>[2x]FACKTANGTAIPIGGGSANVYVNLAPAVNVGQNLVVDLSTQIFCHNDYPETITDYVTLQRGSAYGGVLSSFSGTVKYNGSSYPFPTTSETPRVVYNSRTDKPWPVALYLTPVSSAGGVAIKAGSLIAVLIL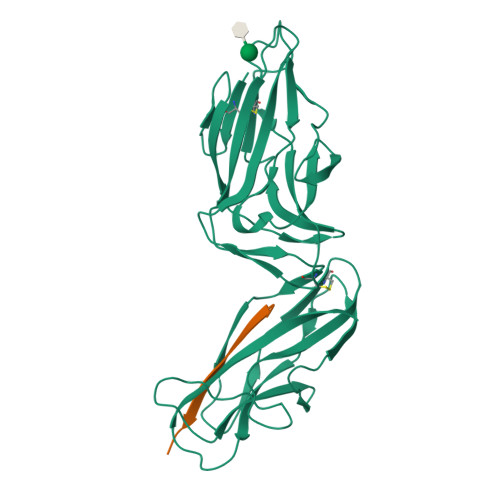RQTNNYNSDDFQFVWNIYANNDVVVPTGGCDVSARDVTVTLPDYPGSVPIPLTVYCAKSQNLGYYLSGTTADAGNSIFTNTASFSPAQGVGVQLTRNGTIIPANNTVSLGAVGTSAVSLGLTANYARTGGQVTAGNVQSIIGVTFVYQ;>ADVTITVNGKVVAK[2x]> MGANASALEKEIGPEQFPVNEHYFGLVNFGNTCYCNSVLQALYFC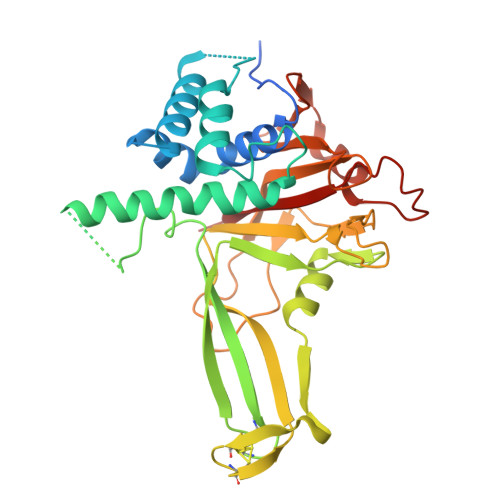RPFREKVLAYKSQPRKKESLLTCLADLFHSIATQKKKVGVIPPKKFITRLRKENELFDNYMQQDAHEFLNYLLNTIADILQEERKQEKQNGRLPNGNIDNENNNSTPDPTWVHEIFQGTLTNETRCLTCETISSKDEDFLDLSVDVEQNTSITHCLRGFSNTETLCSEYKYYCEECRSKQEAHKRMKVKKLPMILALHLKRFKYMDQLHRYTKLSYRVVFPLELRLFNTSGDATNPDRMYDLVAVVVHCGSGPNRGHYIAIVKSHDFWLLFDDDIVEKIDAQAIEEFYGLTSDISKNSESGYILFYQSRD> MKTNLKNNIMKGMAVMPFLSVCVGVAAQQKQMNVIYIMSDDHTSQAIGAYGSRLAVLNPTPTIDELARDGMLFENCFCTNSISTPSRACIMTGQYSHRNKVLTLDEVLQPDQEYLVDEFHNMGYQTAMIGKWHLGCEPSHFDYYSVFNGHGGQGEYFDPTFLTSDVTDKKWPNNQIKKMGYSSDIVTNLAIDWLKNRRDKSKPFFMMHHYKAPNDMFEYAPRYEYYLDDVEV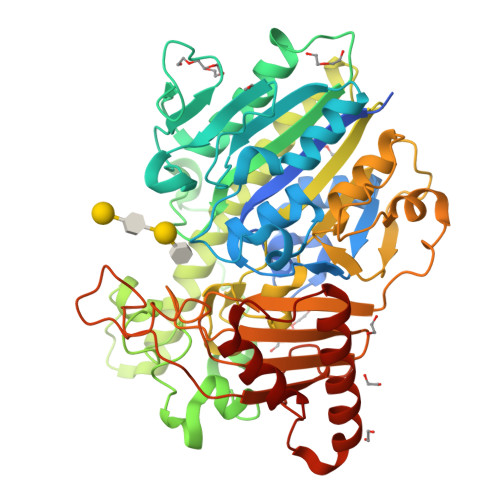PVPLSLFDTDKWGSEGTRGKNDSLRHFIGTSVSSRHEIRNYVMEYKCNTGDEMENTYLAYQHYLKSYLRCVKGVDDNLKRLFDYLKKEGLWENTIIVYTGDQGMMLGEHDLQDKRWMYEESQRMPFIVRDPRCPYKGAKSDLMINNIDFAPTLIEMVGGKEPSYMDGKSFASVFEGKKPENWKDAVYYRYWMHMIHHDVPAHIGIRTENYKLILFYGRHYDDKRYGQKSMSWLKNSHKIVPTLVSFELYDVKNDPYEMVNLADNPKYAKVLKDMKKKLRELRKQVGDTDEAYPELKKVIDKALR>MLLTPEKLLEAANKQGTVPSRVRYQWMEDEETGRLKAVGYHTSMESGRDQVRVRLLKHDFPNNRYEFWEEGATGPTILWTPD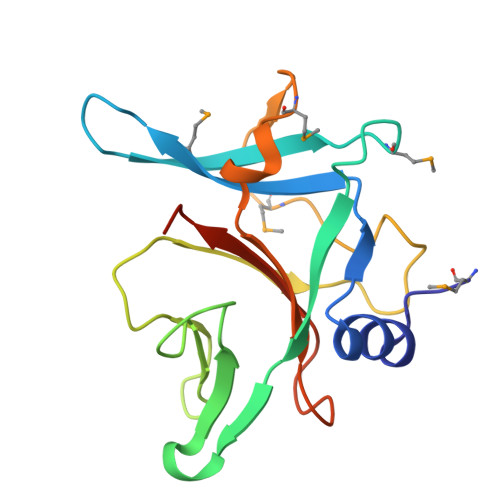NPGIELPTDTAHGEQPVIPSAIPGLEIPEMDDVSILATPMPDEKDFRDYILVFPENAFPPIYVYLSKLEHHHHHH[4x]4-[3-(1-methylethyl)-1H-pyrazol-4-yl]-N-(1-methylpiperidin-4-yl)pyrimidin-2-amine 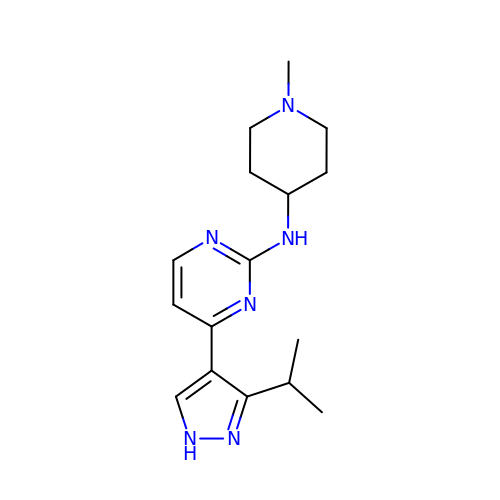| C16 H24 N6 | YVKZWLZGQQCODL-UHFFFAOYSA-N>[2x]MPAIVCQSALEAVSLIRSGETLWTHSMGATPKVLLDALAKHALT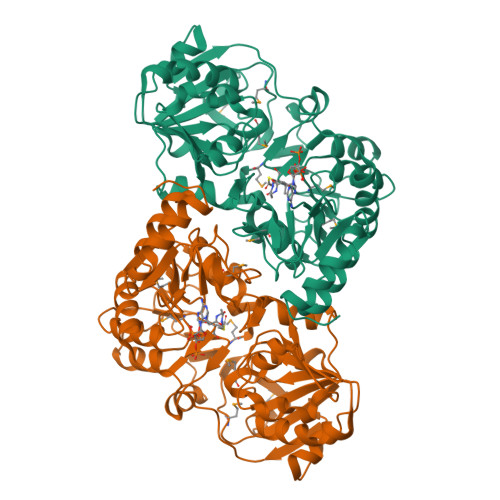LDNITLLQLHTEGAESLSHPSLLGHLRHRCFFGGVPTRPLLQSGDADYVPIFLSEVPKLFRSGEQKIDTAIIQVSPPDKHGMCSLGISVEATLAACQVAGKIIAHINPQMPRTHGDGFIHIDRFAAVYEQSASLPIHSFATGDAVSLAIGQHVAELVRDGDCLQMGIGAIPDAVLSCLTGHKDLGVHTELFSDGILQLVEKGVINNTKKRFYPGKLVTGFALGSQKLYDYVDDNPAVIFMDIEQVNDTSIIRKNPNVMAINSALQVDLTGQVCADSIGTKIYSGVGGQMDFIRGAGLSEGGRSVIALPSTAAGGRISRIASVLSPGAGVVTTRAHVHYIVTEYGAANLKGRSLRERAQALINIAHPDFREQLSRDAFEVWGLNLLEHHHHHH> LTGEFEKKYVA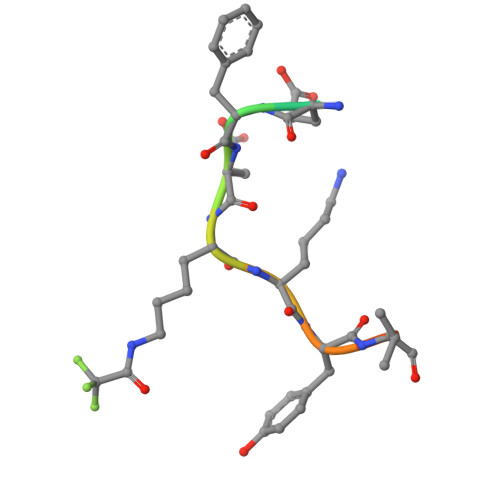TL> DTATGIPVVNDST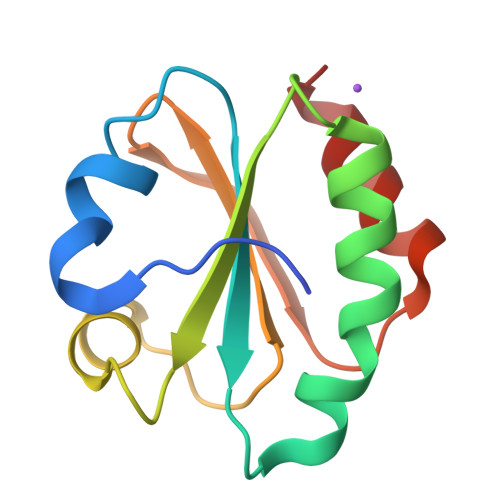WDSLVLKADEPVFVDFWAPWCGPSKMIDPIVNELAQKYAGQFKFYKLNTDESPATPGQYGVRSIPTIMIFVNGEKKDTIIGAVSKDTLATSINKFL2-KETO-3-DEOXYGLUCONATE | C6 H10 O6 | 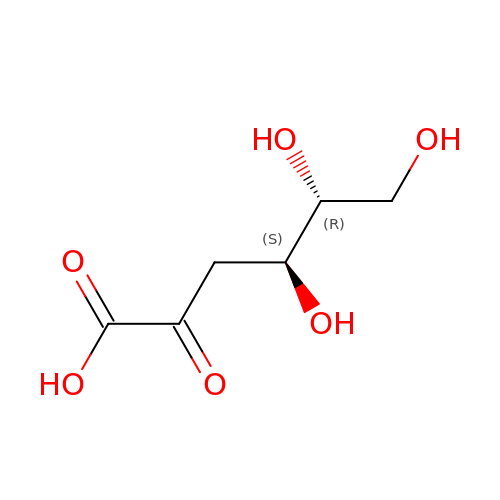WPAMZTWLKIDIOP-WVZVXSGGSA-N> VEPP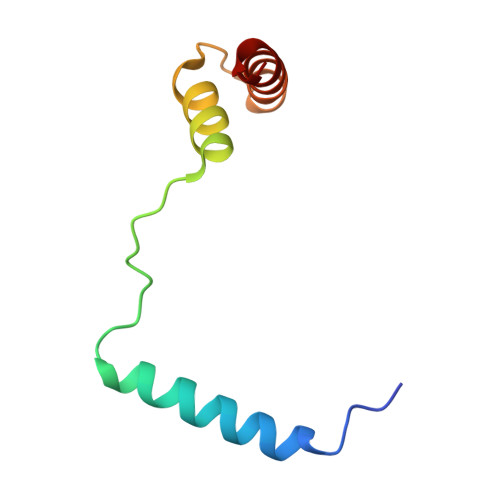PDDYLMKLQKQLASFQSILESGDLSINKAVENEEITLISKALKESTIVEPIERGVAALIAFHGQNE> SISSRVKSKRIQLGLNQAELAQKVGTTQ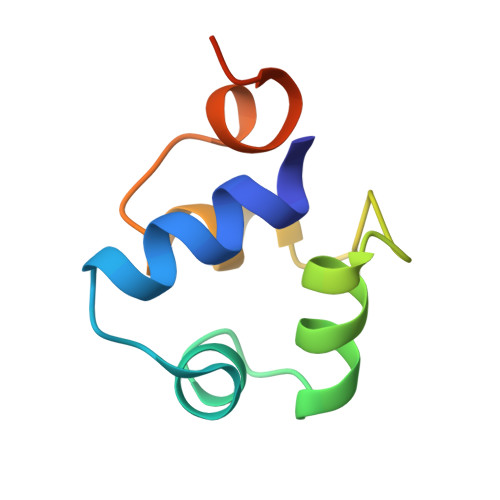QSIEQLENGKTKRPRFLPELASALGVSVDWLLNGTSDSNVR>ALEKDRRALEALKRAQEAEKKGDVEEAVRAAQEAVRAA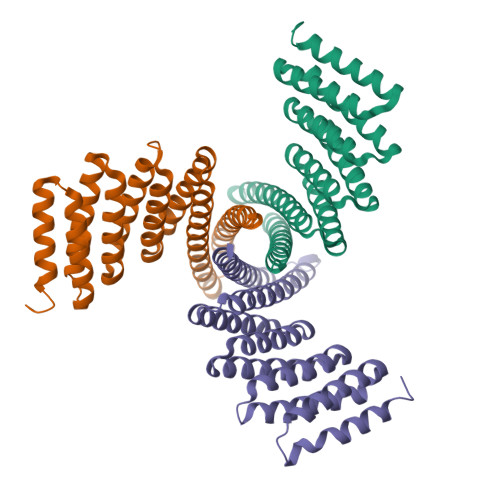KESGASWILRLVAEQALRIAKEAEKQGNVEVAVKAARVAVEAAKQAGDNDVLRKVAEQALRIAKEAEKQGNVDVAAKAAQVAAEAAKQAGDKDMLEKVAKVAEQIAKAAEKEGDKKVSIDATRIALEASLAALEIILEELKEMLERLEKNPDKDVIVKVLKVIVKAIEASVKNQKISAKNQKALAELA[6x]>MPRFSNKTVIITGSSNGIGRTTAILFAQEGANVTITGRSSERLEETRQIILKSGVSEKQVNSVVADVTTEDGQDQIINSTLKQFGKIDVLVNNAGAAIPDAFGTTGTDQGIDIYHKTLKLNLQAVIEMTKKVKPHLVASKGEIVNVSSIVAGPQAQPDFLYYAIAKAALDQYTRSTAIDLAKFGIRVNSVSPGMVETGFTNAMGMPDQASQKFYNFMASHKECIPIGAAGKPEHIANIILFLADRNLSFYILGQSI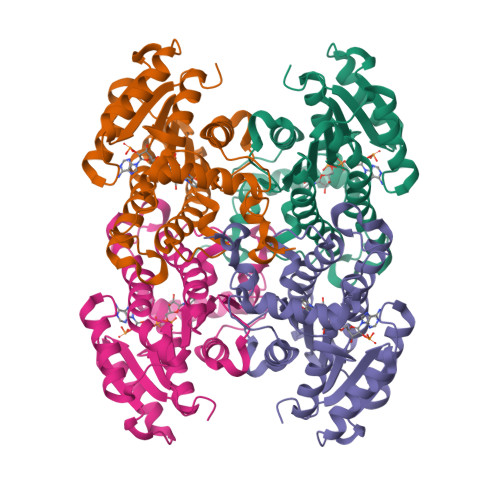VADGGTSLVMGTQAHDVMSIMSSH[4x]> MHHHHHHSSGRENLYFQGETSVPPGSALVGPSCVMDDFRDPQRWKECAKQGKMPCYFDLIEENVYLTERKKNKSHRDIKRMQCECTPLSKDERAQGEIACGEDCLNRLLMIECSSRCPNGDYCSNRRFQRKQHADVEVILTEKKGWGLRAAKDLPSNTFVLEYCGEVLDHKEFKARVKEYARNKNIHYYFMALKNDEIIDATQKGNCSRFM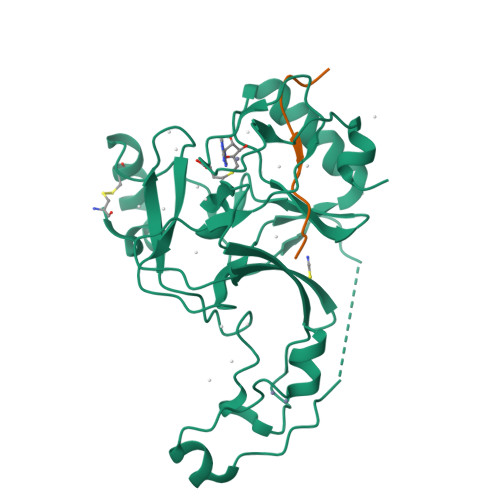NHSCEPNCETQKWTVNGQLRVGFFTTKLVPSGSELTFDYQFQRYGKEAQKCFCGSANCRGYLGGENRVSIRAAGGKMKKERSRK;> APRFGGVMRPNRYR> GSHMASMTGGQQMGRGSWKRAFLAFGSNIGDRFKHIQMALQLLSREKTVKLRNISSIFESEPMYFKDQTPFMNGCVEVETLLTPSELLKLCKKIEYEELQRVKHFDNGPRTIDLDIVMFLNSAGEDIIVNEPDLNIPHPRMLERTFVLEPLCELISPVHLHPVTAEPIVDHLKQLYDKQHDEDTLWKLVPLPYRSGVEPRFLKFKTATKLDEFTGETNRITVSPTYIMAIFNATPDSFSDGGEHFADIESQLNDIIKLCKDALYLHESVIIDVGGCSTRPNSIQASEEEEIRRSIPLIKAIRESTELPQDKVILSIDTYRSNVAKEAIKVGVDIINDISGGLFDSNMFAVIAENPEICYILSHTRGDISTMNRLAHYENFALGDSIQQEFVHNTDIQQLDDLKDKTVLIRNVGQEIGERYIKAIDNGVKRWQILIDPGLGFAKTWKQNLQIIRHIPILKNYSFTMNSNNSQVYVNLRNMPVLLGPSRKKFIGHITKDVDAKQR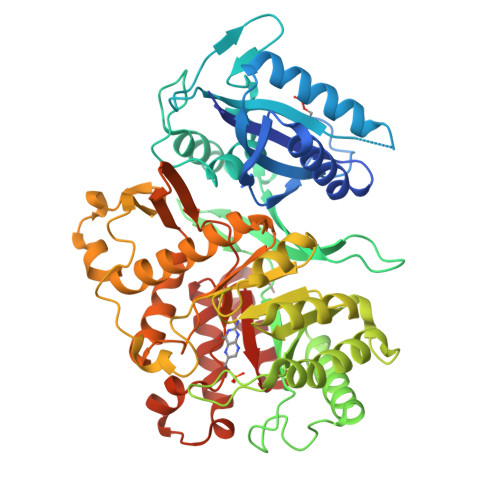DFATGAVVASCIGFGSDMVRVHDVKNCSKSIKLADAIYKGLE> MESTA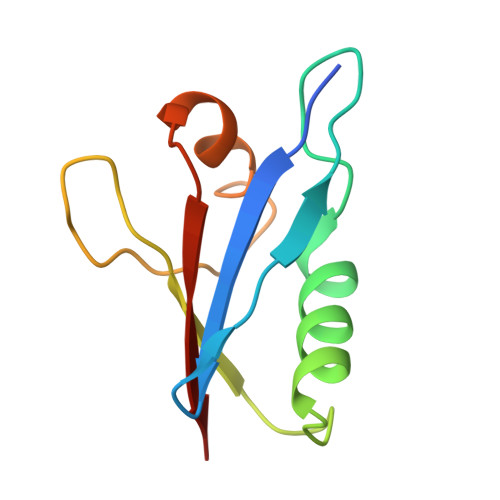NALVVKVSYGGVLRRFRVPVKANGQLDLEMAGLKEKIAALFNLSADAELSLTYSDEDGDVVALVDDNDLFDVTNQRLKFLKINVNAGVS> SMDF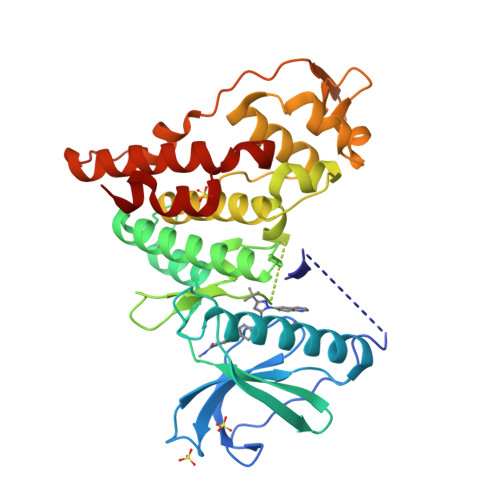KENPNLRDNWTDAEGYYRVNIGEVLDKRYNVYGYTGQGVFSNVVRARDNARANQEVAVKIIRNNELMQKTGLKELEFLKKLNDADPDDKFHCLRLLRHFYHKQHLCLVFEPLSMNLREVLKKYGKDVGLHIKAVRSYSQQLFLALKLLKRCNILHADIKPDNILVNESKTILKLCDFGSASHVADNDITPYLFSRFYRAPEIIIGKSYDYGIDMWSVGCTLYELYTGKILFPGKTNNHMLKLAMDLKGKMPNKMIRKGVFKDQHFDQNLNFMYIEVDKVTEREKVTVMSTINPTKDLLADLIGCQRLPEDQRKKVHQLKDLLDQILMLDPAKRISINQALQHAFIQE>GSFSKEESREFMAIFPDIVRDLTDAGRHTDIPEVTKRFAKVLQYNVPTGKKTRGLSTVIAYKMLEKPENLTPENVRLAGILGWCVELLQASLLIMDDLMDRSETRRGQPCWYRQENVGFLAINDCLHVESSLYSVLRKYFSHLPCYVPIIELFHDVNFKTNMGQSLDALCMKDGRPILSQFTMKRYSSIVKYKTSYYTFQLPVSLGMYLADMYDPEQHRQAKTILMEIGEFFQIQDDFLDAFGDSQVTGKVGTDIKEGKCSWLAVVALQRSNPAQRQIMEEHYGRPEPESTQIIKNLYIELGLPATFAVYEEESFNIIRTHIHQISKGLPHDLFFKIMKKIYKRDA[2x]

Here we characterize a metal-dependent, bifunctional isoprenyl diphosphate synthase from the leaf beetle Phaedon cochleariae by structural and functional analyses. Isoprenyl diphosphate synthase in P. cochleariae (PcIDS1, EC 2.5.1.1) produces FPP in the presence of Mg2+, but preferably forms GPP when exposed to the heavy metal ions (HMIs) Co2+ or Mn2+. Inter- and intramolecular cooperative effects in the homodimer strongly depend on the provided metal ions and regulate the biosynthetic flux of terpene precursors to either biological defence or physiological development. Strikingly, a unique chain length determination domain adapts to form geranyl or farnesyl pyrophosphate by altering enzyme symmetry and ligand affinity between both subunits.

Each subunit (subA and subB) consists of 13 helices (αA to αJ and α1 to α3). In both chains, the N terminus and C terminus as well as the loops between αD–αE (183–201) and αH–α1 (329–332) are disordered. The FARM region (179–183) is partially resolved, while D319 of the SARM (319–323) coordinates a pentahydrated Mg2+ at site B (Mg2+B).> AIGEFMVSLPRMVYPQPKVLTPCRKDVLVVTPWLAPIVWEGTFNIDILNEQFRLQNTTIGLTVFAIKKYVAFLKLFLETAEKHFMVGHRVHYYVFTDQPAAVPRVTLGTGRQLSVLEVRAYKRWQDVSMRRMEMISDFCERRFLSEVDYLVCVDVDMEFRDHVGVEILTPLFGTLHPSFYGSSREAFTYERRPQSQAYIPKDEGDFYYMGAFFGGSVQEVQRLTRACHQAMMVDQANGIEAVWHDESH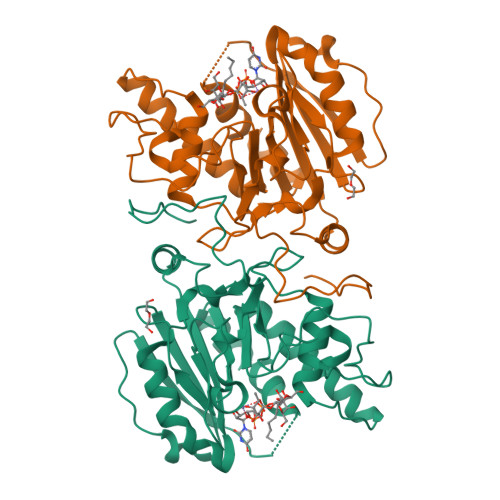LNKYLLRHKPTKVLSPEYLWDQQLLGWPAVLRKLRFTAVPKNHQAVRNPE> GMSADIVFDRGSPSDIDEIKTFTSNTWKVGYYTDLYSKLADTGTMDDYVDKVIERWVNDGSVYVLRVSGRPVATIHMEKLPDGSVMLGGLRVHPEYRGSRLGMSIMQETIQFLRGKTERLRSAVYSWNEPSLRLVHRLG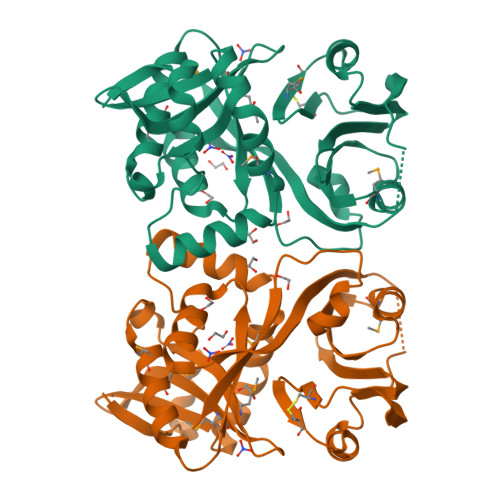FHQVEEYPIYTFQGGSTAVPALKPVNERYAGRWRCFFIDWKYMCSDDPDIIHEEYSNNLIVDGSTFVYFDIYEGGIDLFVNDSDDASSFIEKYRSMNGRITFYVRKALANGLPYVPASSLTVWEYRY> MAGSATVEKRLDFGLLGPLQMTIDGTPVPSGTPKQRAVLA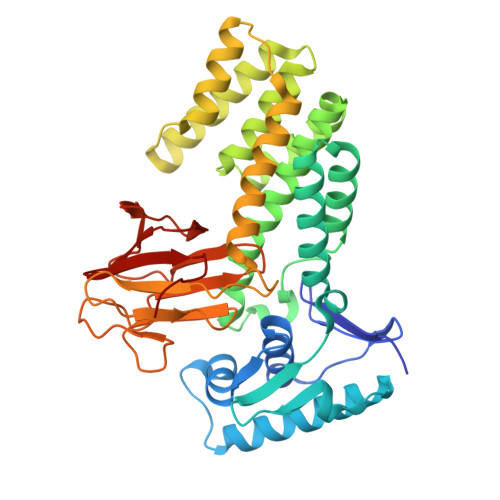MLVINRNRPVGVDALITALWEEWPPSGARASIHSYVSNLRKLLGGAGIDPRVVLAAAPPGYRLSIPDNTCDLGRFVAEKTAGVHAAAAGRFEQASRHLSAALREWRGPVLDDLRDFQFVEPFATALVEDKVLAHTAKAEAEIACGRASAVIAELEALTFEHPYREPLWTQLITAYYLSDRQSDALGAYRRVKTTLADDLGIDPGPTLRALNERILRQQPLDAKKSAKTTAAGTVTVLDQRTMASGQQAVAYLHDIASGRGYPLQAAATRIGRLHDNDIVLDSANVSRHHAVIVDTGTNYVINDLRSSNGVHVQHERIRSAVTLNDGDHIRICDHEFTFQISAGTHGGT> MPPGVDCPMEFWTKEENQSVVVDFLLPTGVYLNFPVSRNANLSTIKQLLWHRAQYEPLFHMLSGPEAYVFTCINQTAEQQELEDEQRRLCDVQPFLPVLRLVAREGDRVKKLINSQISLLIGKGLHEFDSLCDPEVNDFRAKMCQFCEEAAARRQQLGWEAWLQYSFPLQLEPSAQTWGPGTLRLPNRALLVNVKFEGSEESFTFQVSTKDVPLALMACALRKKATVFRQPLVEQPEDYTLQVNGRHEYLYGSYPLCQFQYICSCLHSGLTPHLTMVHSSSILAMRDEQSNPAPQVQKPRAKPPPIPAKKPSSVSLWSLEQPFRIELIQGSKVNADERMKLVVQAGLFHGNEMLCKTVSSSEVSVCSEPVWKQRLEFDINICDLPRMARLCFALYAVIEKAKKARSTKKKSKKADCPIAWANLMLFDYKDQLKTGERCLYMWPSVPDEKGELLNPTGTVRSNPNTDSAAALLICLPEVAPHPVYYPALEKILELGRHSECVHVTEEEQLQLREILERRGSGELYEHEKDLVWKLRHEVQEHFPEALARLLLVTKWNKHEDVAQMLYLLCSWPELPVLSALELLDFSFPDCHVGSFAIKSLRKLTDDELFQYLLQLVQVLKYESYLDCELTKFLLDRALANRKIGHFLFWHLRSEMHVPSVALRFGLILEAYCRGSTHHMKVLMKQGEALSKLKALNDFVKLSSQKTPKPQTKELMHLCMRQEAYLEALSHLQSPLDPSTLLAEVCVEQCTFMDSKMKPLWIMYSNEEAGSGGSVGIIFKNGDDLRQDMLTLQMIQLMDVLWKQEGLDLRMTPYGCLPTGDRTGLIEVVLRSDTIANIQLNKSNMAATAAFNKDALLNWLKSKNPGEALDRAIEEFTLSCAGYCVATYVLGIGDRHSDNIMIR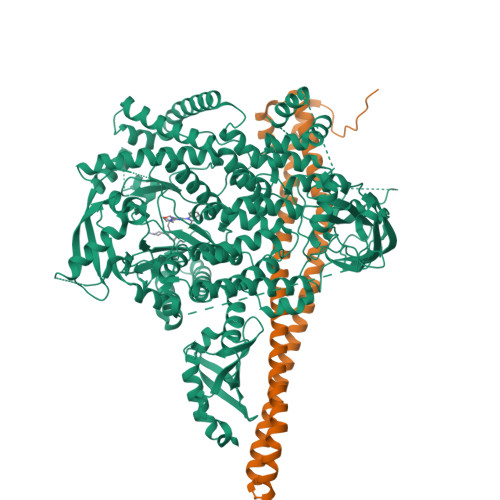ESGQLFHIDFGHFLGNFKTKFGINRERVPFILTYDFVHVIQQGKTNNSEKFERFRGYCERAYTILRRHGLLFLHLFALMRAAGLPELSCSKDIQYLKDSLALGKTEEEALKHFRVKFNEALRESWKTKVNWLAHNVSKDNRQ;> XMYQQDQVVKEDNIEAVGKKLHEYNTQFQEKSREYDRLYEDYTRTSQEIQMKRTAIEAFNETIKIFEEQCQTQERYSKEYIEKFKREGNETEIQRIMHNYEKLKSRISEIVDSRRRLEEDLKKQAAEYREIDKRMNSIKPDLIQLRKTRDQYLMWLTQKGVRQKKLNEWLGN> VLGGGAIYGGGSRCSAAFNVTKGGARYFVTAGHCTNISANWSASSGGSVVGVREGTSFPTNDYGIVRYTDGSSPAGTVDLYNGSTQDISSAANAVVGQAIKKSGSTTKVTSGTVTAVNVTVNYGDGPVYNMVRTTACSAGGDSGGAHFAGSVALGIHSGSSGCSGTAGSAIHQPVTEALSAYGVTVY;>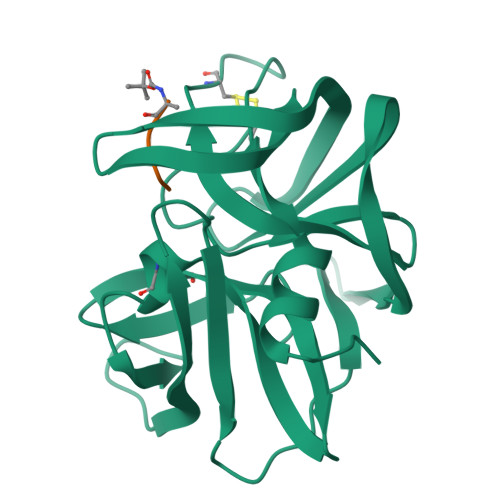 XAAPE> MDKKGSDSGKASGEQVLNLTESALIPSADSTKADDQVGLNVVNQTNEGLYALDKDGIPAIAGAAEEPKISDDKTVYTIKLREDAKWSNGDPVTANDYVYSWRRAVDPNTAATYSYLFDAIKNGGDIVAGKKKPEELGIKAVDDYTLEVTLSKPTAYINSLFAFPTFFPLNEKFVTEKGEKYAQNSDNMLFNGPFELKDWTGTNKKWTYVKNDKYWDKDKVKLKQINVQVVQDSGTGLNLYNTDKVDRTVLSADYAAQNKNNKDYVTVNNSSTFYIKFNQKRAGKDTVFANKNIRKAIALAIDKQSYTDTVLKNGSKPANNLVPEGFTF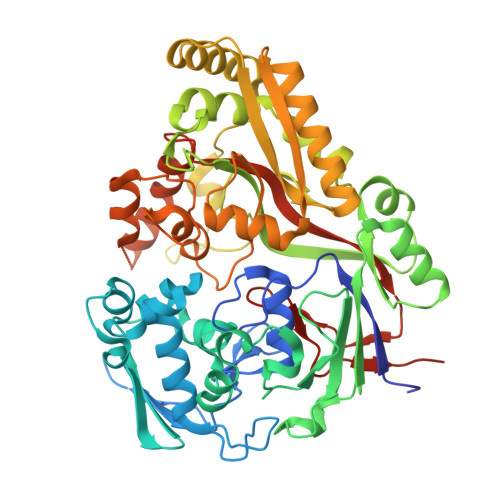DPGNKEDYTKESGKHLEYDVKEAQKAWKAGLKELGVNEITVEFTSDDTENARKSSEFIQDQLQKNLDGLTVKLKNVPFKVRLQNDQNQDYDFSMSGWGPDYQDPSTFLDLFVTDGAQNRMSYSNKDYDKILNDASVTYAADDQKRWDEMVKAEKILLTDDVAIQPLYQRSTAYLQKDYIKNLQKNPFGPDYTYKETYLTKLEHHHHHH>[2x]MVTVGNYCEAEGPVGPAWMQDGLSPCFFFTLVPSTRMA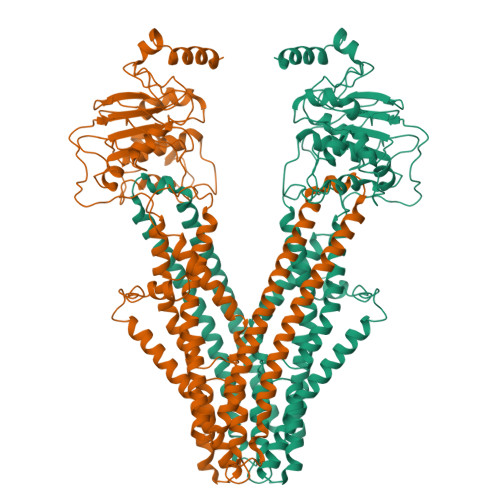LGTLALVLALPCRRRERPAGADSLSWGAGPRISPYVLQLLLATLQAALPLAGLAGRVGTARGAPLPSYLLLASVLESLAGACGLWLLVVERSQARQRLAMGIWIKFRHSPGLLLLWTVAFAAENLALVSWNSPQWWWARADLGQQVQFSLWVLRYVVSGGLFVLGLWAPGLRPQSYTLQVHEEDQDVERSQVRSAAQQSTWRDFGRKLRLLSGYLWPRGSPALQLVVLICLGLMGLERALNVLVPIFYRNIVNLLTEKAPWNSLAWTVTSYVFLKFLQGGGTGSTGFVSNLRTFLWIRVQQFTSRRVELLIFSHLHELSLRWHLGRRTGEVLRIADRGTSSVTGLLSYLVFNVIPTLADIIIGIIYFSMFFNAWFGLIVFLCMSLYLTLTIVVTEWRTKFRRAMNTQENATRARAVDSLLNFETVKYYNAESYEVERYREAIIKYQGLEWKSSASLVLLNQTQNLVIGLGLLAGSLLCAYFVTEQKLQVGDYVLFGTYIIQLYMPLNWFGTYYRMIQTNFIDMENMFDLLKEETEVKDLPGAGPLRFQKGRIEFENVHFSYADGRETLQDVSFTVMPGQTLALVGPSGAGKSTILRLLFRFYDISSGCIRIDGQDISQVTQASLRSHIGVVPQDTVLFNDTIADNIRYGRVTAGNDEVEAAAQAAGIHDAIMAFPEGYRTQVGERGLKLSGGEKQRVAIARTILKAPGIILLDEATSALDTSNERAIQASLAKVCANRTTIVVAHRLSTVVNADQILVIKDGCIVERGRHEALLSRGGVYADMWQLQQGQEETSEDTKPQTMERDYKDDDDK3-[(2-chlorophenyl)methylamino]pyrazine-2-carboxamide | C12 H11 Cl N4 O | 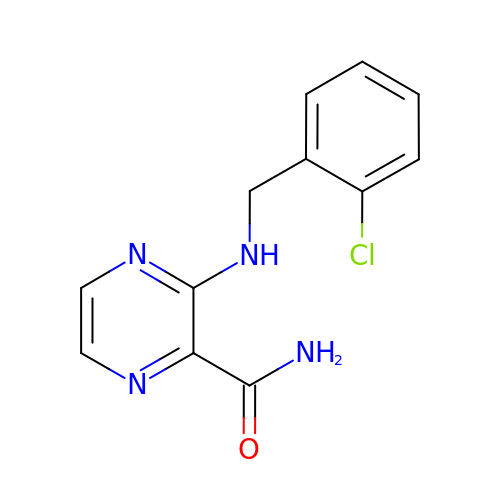SZIKCJPPVPPUMU-UHFFFAOYSA-N> GSNRRLQQTQ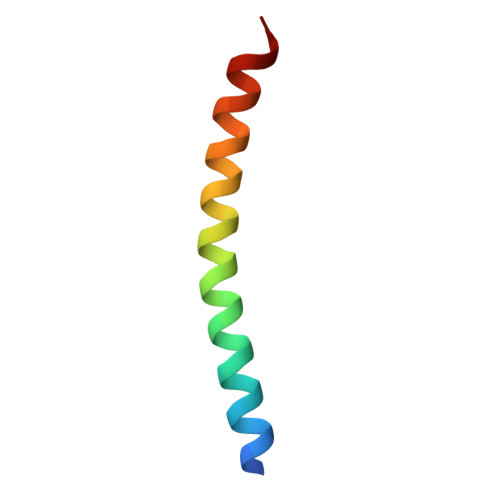AQVDEVVDIMRVNVDKVLERDQKLSELDDR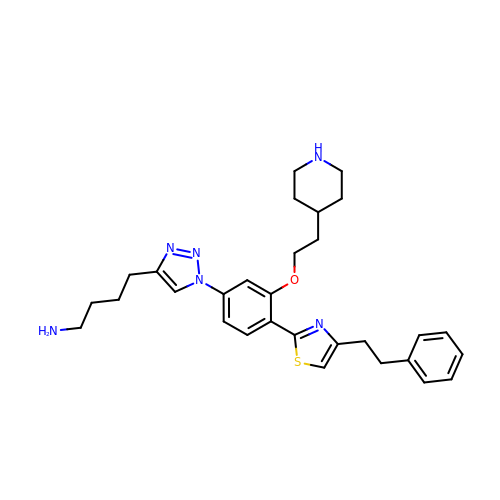4-[1-[4-[4-(2-phenylethyl)-1,3-thiazol-2-yl]-3-(2-piperidin-4-ylethoxy)phenyl]-1,2,3-triazol-4-yl]butan-1-amine | C30 H38 N6 O S | YMQYETVMOWEEHG-UHFFFAOYSA-N>WVQPITCQKPSLTLWLDDKMFTGLINTGADVTIIKLEDWPPNWPITDTLTNLRGIGQSNNPKQSSKYLTWRDK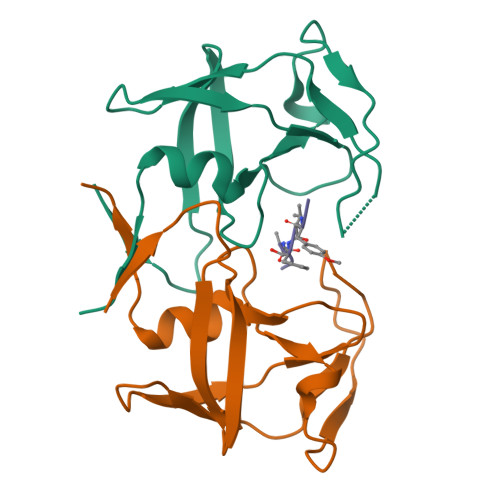ENNSGLIKPFVIPNLPVNLWGRDLLSQMKIMMCSPNDIVTA[2x];> PYVFAMT> 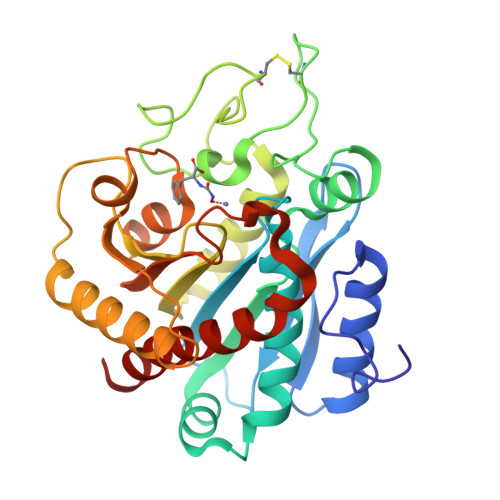ARSTNTFNYATYHTLDEIYDFMDLLVAEHPQLVSKLQIGRSYEGRPIYVLKFSTGGSNRPAIWIDLGIHSREWITQATGVWFAKKFTEDYGQDPSFTAILDSMDIFLEIVTNPDGFAFTHSQNRLWRKTRSVTSSSLCVGVDANRNWDAGFGKAGASSSPCSETYHGKYANSEVEVKSIVDFVKDHGNFKAFLSIHSYSQLLLYPYGYTTQSIPDKTELNQVAKSAVEALKSLYGTSYKYGSIITTIYQASGGSIDWSYNQGIKYSFTFELRDTGRYGFLLPASQIIPTAQETWLGVLTIMEHTLNN>[3x]SIGERPVLKAPAPKRQKCDHWSPCPPDTYAYRLLSGGGR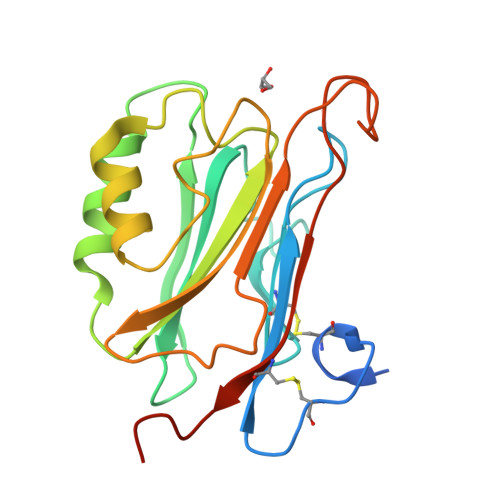DKYAKICFEDEVLIGEKTGNVARGINIAVVNYETGKVIATKYFDMYEGDNSGPMAKFIQSTPSKSLLFMVTHDDGSSKLKAQAKDAIEALGSKEIKNMKFRSSWVFVAAKGFELPSEIEREKINHSDQSRNRYAGWPAEIQIEGCIPKGLRDYKDDDDK>[8x]MADPLTPAISDRICKHMNEDHASAIALYAQVFGQQTDVTMAQMQAIDPTGMDLVV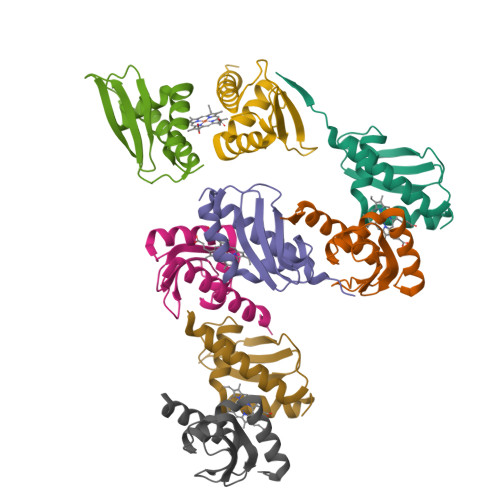ESEGGSKTIRIEFEQPLKDSEDAAQVLIAMAKQAASVGKNSAENLYFQ>PPYTVVYFPVRGRCAALRMLLADQGQSWKEEVVTVETWQEGSLKASCLYGQLPKFQDGDLTLYQSNTILRHLGRTLGLYGKDQQEAALVDMVNDGVEDLRCKYISLIYTNYEAGKDDYVKALPGQLKPFETL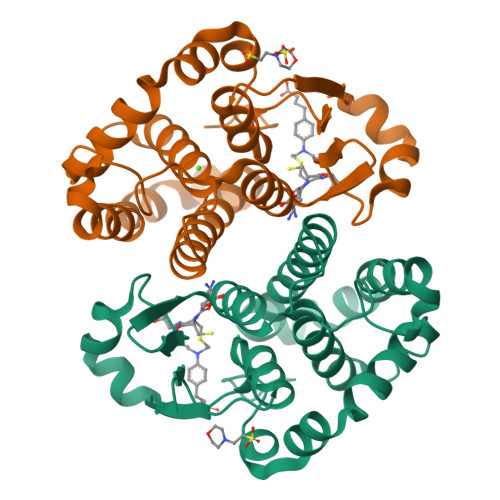LSQNQGGKTFIVGDQISFADYNLLDLLLIHEVLAPGCLDAFPLLSAYVGRLSARPKLKAFLASPEYVNLPINGNGKQ[2x]>[2x]LEDVVIDRNLLILGKILGEGEFGSVMEGNLKQEDGTSLKVAVKTMKLDNSSQREIEEFLSEAACMKDFSHPNVMRLLGVCIEMSSQGIPKPMVILPFMKYGDLHTYLLYSRLETGPKHIPLQTLLKFMVDIALGMEYLSNRNFLHRDLAARNCMLRDDMTVCVADFGLSKKIYSGDYYRQGRIAKMPVKWIAIESLADRVYTSKSDVWAFGVTMWEIATRGMTPYPGVQNHEMYDYLLH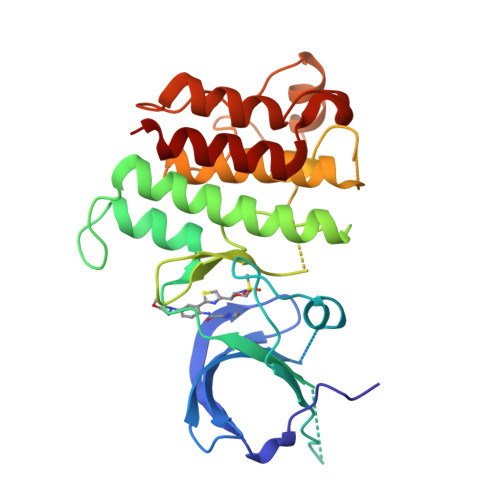GHRLKQPEDCLDELYEIMYSCWRTDPLDRPTFSVLRLQLEKLLESL> MSAVEISPDVLVYKSPLTEQSTEYASISNNSDQTIAFKVKTTAPKFYCVRPNAAVVAPGETIQVQVIFLGLTEEPAADFKCRDKFLVITLPSPYDLNGKAVADVWSDLEAEFKQQAIS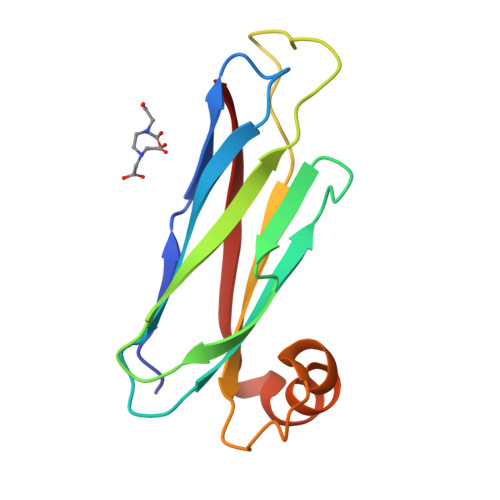KKIKVKYL>[2x]MPMVLLECDKDIPERQKHIYLKAPNEDTREFLPIANAATIPGTLSERGCAFCGAKLVIGGVLKDTIQMIHGPLGCAYDTWHTKRYPTDNGHFNMKYVWSTDMKESHVVFGGEKRLEKSMHEAFDEMPDIKRMIVYTTCPTALIGDDIKAVAKKVMKDRPDVDVFTVECPGFSGVSQSKGHHVLNIGWINEKVETMEKEITSEYTMNFIGDFNIQGDTQLLQTYWDRLGIQVVAHFTGNGTYDDLRCMHQ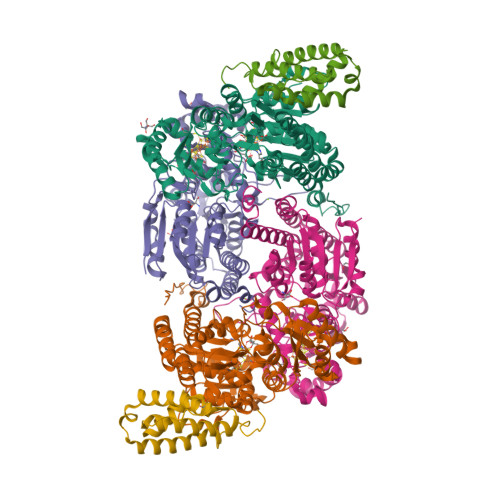AQLNVVNCARSSGYIANELKKRYGIPRLDIDSWGFNYMAEGIRKICAFFGIEEKGEELIAEEYAKWKPKLDWYKERLQGKKMAIWTGGPRLWHWTKSVEDDLGVQVVAMSSKFGHEEDFEKVIARGKEGTYYIDDGNELEFFEIIDLVKPDVIFTGPRVGELVKKLHIPYVNGHGYHNGPYMGFEGFVNLARDMYNAVHNPLRHLAAVDIRDKSQTTPVIVRGAA;>[2x]MSNCELTVLKPAEVKLSPRDREGIINPMYDCQPAGAQYAGIGIKDCIPLVHGGQGCTMFVRLLFAQHFKENFDVASTSLHEESAVFGGAKRVEEGVLVLARRYPNLRVIPIITTCSTEVIGDDIEGSIRVCNRALEAEFPDRKIYLAPVHTPSFKGSHVTGYAECVKSVFKTITDAHGKGQPSGKLNVFPGWVNPGDVVLLKRYFKEMDVEANIYMDTEDFDSPMLPNKSIETHGRTTVEDIADSANALATLSLARYEGNTTGELLQKTFAVPNALVNTPYGIKNTDDMLRKIAEVTGKEIPESLVRERGIALDALADLAHMFFANKKVAIFGHPDLVLGLAQFCMEVELEPVLLLIGDDQGNKYKKDPRIEELKNTAHFDIEIVHNADLWELEKRINAGLQLDLIMGHSKGRYVAIEANIPMVRVGFPTFDRAGLYRKPSIGYQGAMELGEMIANAMFAHMEYTRNKEWILNTW;>MSQSHLDDLFAYVEERCLWQFFSRTWDREENIEGVLNQVGRLLTGQEPLRGTPQERLFYADALAMANDVRERFPWASQVNKEEIEFLLDGLKSRLVDVTITRSTNRELNHHLY[2x]> SNAGSSDEKTLTVSVDAGYKDYVNKIKGDFEKDNDVKVKVVEKDMFETLEALPLDGPAGTAPDVMMSAFDRIGSLGQQGHLAEVKLGNKDDYDEKDQKQVTIDDKIYGAPAIIETLVLYYNKDLLDKAPATFKDLETLSKDSRFAFTSEKGKNTGFLAKWTDFYFSYGLLAGYGGYVFGDEGTNPKDIGLNNKGSVEGITYATKWFQDVWPKGMQDNKSADDFIQDQFVKGKAAAILGGPWSAANYKEAKINYGVAKIPTLNNGKEYSPFAGGKGWVVSNYSKNKDVAQKWLDYVTNQKNQETLYDMTNEVPANLKARDTAKSKNDELTNAVIEQYKNAQPMPNIPEMSEVWTGA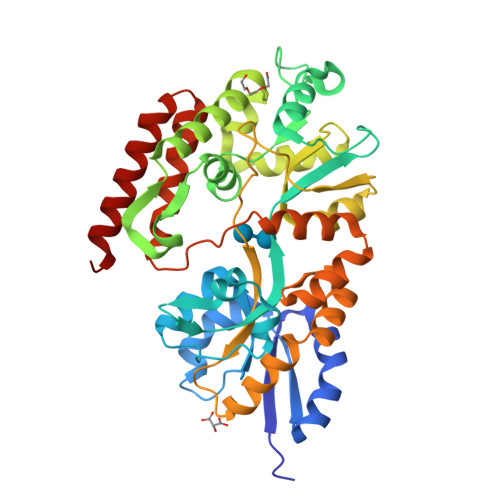ENLKFDAASGSKTPQPSADDAVKVIEDNVTQKYTK> GPLGSMISGIRVNDNCVTEFNNMKIRKTCGWIIFVIQNCEIIIHSKGASTTLTELV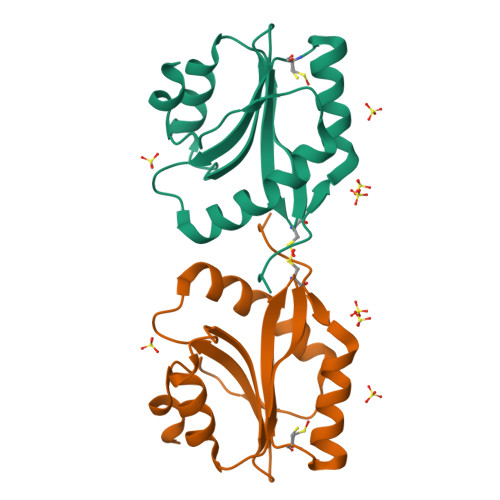QSIDKNNEIQCAYVVFDAVSKIHFFMYARESSNSRDRMTYASSKQAILKKIEGVNVLTSVIESAQDVADLK> HHHHHHKICIGTKSRLSVPSNKEHHYRNLRDRYTNCTYVDGNLELTWLPNENLDLSFLDNIREVTGYILISHVDVKKVVFPKLQIIRGRTLFSLSVEEEKYALFVTYSKMYTLEIPDLRDVLNGQVGFHNNYNLCHMRTIQWSEIVSNGTDAYYNYDFTAPERECPKCHESCTHGCWGEGPKNCQKFSKLTCSPQCAGGRCYGPKPRECCHLFCAGGCTGPTQKDCIACKNFFDEGVCKEECPPMRKYNPTTYVLETNPEGKYAYGATCVKECPGHLLRDNGACVRSCPQDKMDKGGECVPCNGPCPKTCPGVTVLHAGNIDSFRNCTVIDGNIRILDQTFSGFQDVYANYTMGPRYIPLDPERLEVFSTVKEITGYLNIEGTHPQFRNLSYFRNLETIHGRQLMESMFAALAIVKSSLYSLEMRNLKQISSGSVVIQHNRDLCYVSNIRWPAIQKEPEQKVWVNENLRADLCEKNGTICSD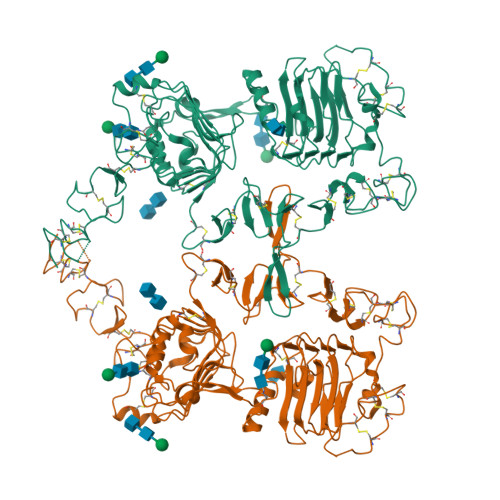QCNEDGCWGAGTDQCLNCKNFNFNGTCIADCGYISNAYKFDNRTCKICHPECRTCNGAGADHCQECVHV>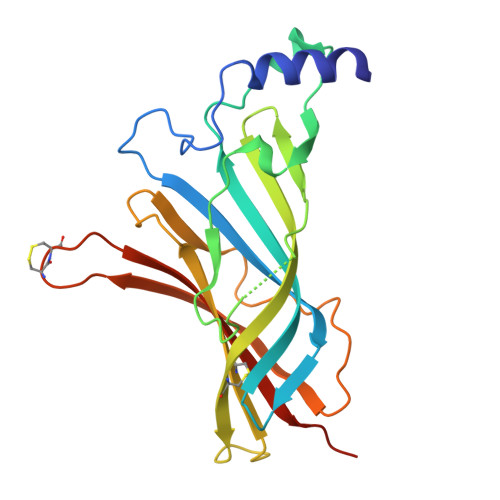 ADGKYAQKLFNDLFEDYSNALRPVEDTDKVLNVTLQITLSQIKDMDERNQILTAYLWIRQIWHDAYLTWDRDQYDGLDSIRIPSDLVWRPDIVLYNKADDESSEPVNTNVVLRYDGLITWDAPAITKSSCVVDVTYFPFDNQQCNLTFGSWTYNGNQVDIFNALDSGDLSDFIEDVEWEVHGMPAVKNVISYGCCSEPYPDVTFTLLLKRRSHHHHHH O-palmitoleoyl serine | C19 H35 N O4 | 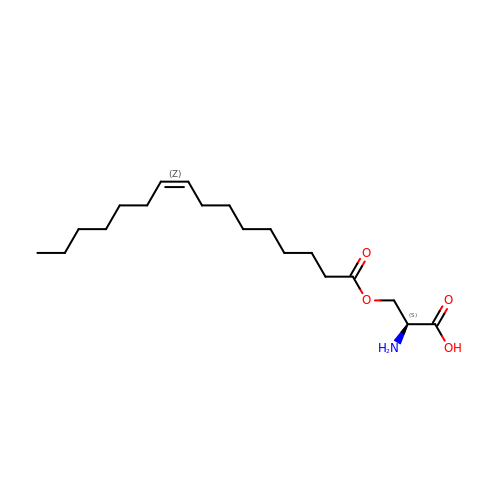BEQLUQLZPXGDLC-QWPQOLDESA-N> GSGSVSSGQAHSLASLAKTWSSGSAKLQRLGPETEDNEGVLLTEKLKPVDYEYREEVHWMTHQPRVGRGSFGEVHRMKDKQTGFQCAVKKVRLEVFRVEELVACAGLSSPRIVPLYGAVREGPWVNIFMELLEGGSLGQLIKQMGC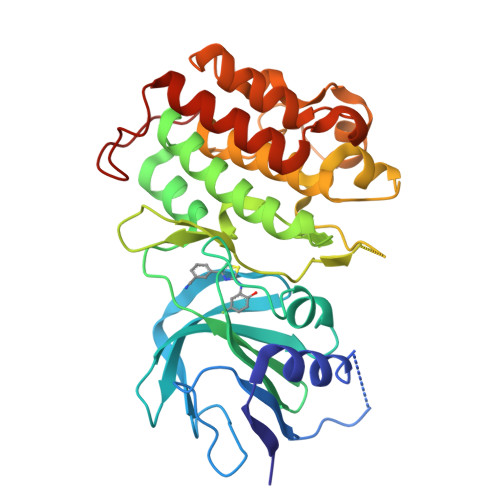LPEDRALYYLGQALEGLEYLHTRRILHGDVKADNVLLSSDGSRAALCDFGHALCLQPDGLGKSLLTGDYIPGTETHMAPEVVMGKPCDAKVDIWSSCCMMLHMLNGCHPWTQYFRGPLCLKIASEPPPIREIPPSCAPLTAQAIQEGLRKEPVHRASAMELRRKVGKALQEVGGLKSPWKGEYKEPRGNS> GHMRKDGFDLDLTYVTDHVIAMSFPSSGRQSLFRNPIGEVSRFFKTKHPDKFRIYNLCSERGYDETKFDNHVYRVMIDDHNVPTLVDLLKFIDDAKVWMTSDPDHVIAIHSKGGKGRTGTLVSSWLLEDGKFDTAKEALEYFGSRRTDFEVGDVFQGVETASQIRYVGYFEKIKKNYGGQLPPMKKLKVTGVTITAIQGVGRGNGSDLSMQIVSERQEVLLCKFAEGYNCAL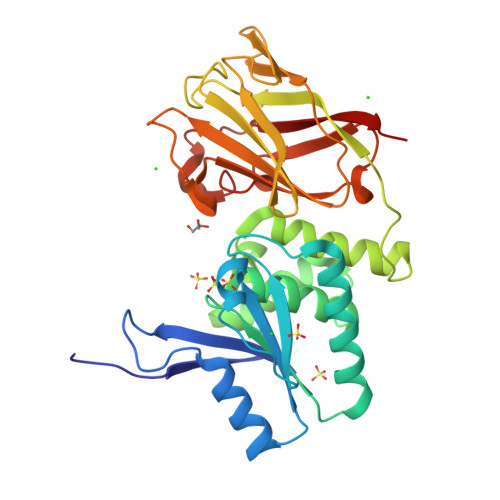QYDATDDCVTCEVKNCPVLAGDIKVRFMSTSKSLPRGYDNCPFYFWFNTSLVEGDHVTLKREEIDNPHKKKTWKIYRDNFTVKLTFSDAEDI>[2x]MGSDKIHHHHHHMYRIRVFGDPVLRKRAKPVTKFDENLKKTIE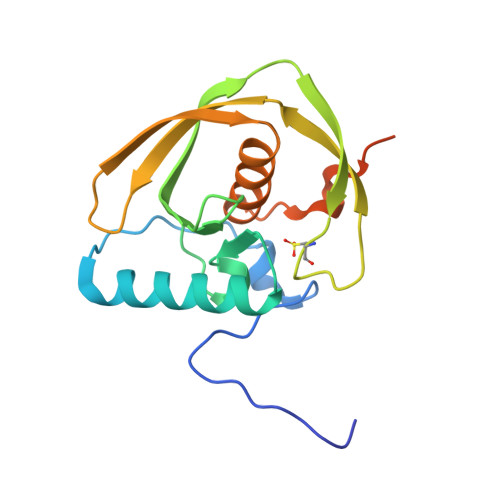RMIETMYHYDGVGLAAPQVGISQRFFVMDVGNGPVAVINPEILEIDPETEVAEEGCLSFPEIFVEIERSKRIKVKYQNTRGEYVEEELEGYAARVFQHEFDHLNGVLIIDRISPAKRLLLRKKLMDIARTVKR> GSHMASDLLEL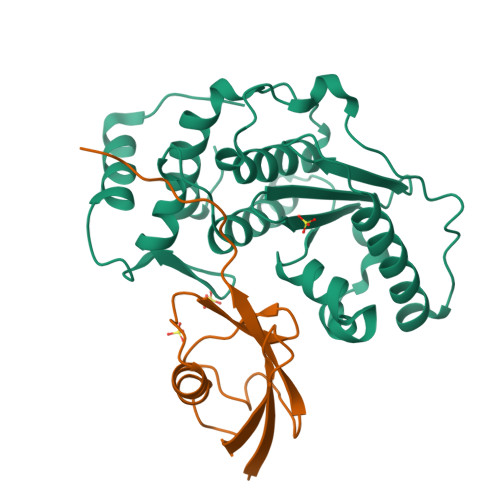TEDMEKEISNALGHGPQDEILSSAFKLRITRGDIQTLKNYHWLNDEVINFYMNLLVERNKKQGYPALHVFSTFFYPKLKSGGYQAVKRWTKGVNLFEQEIILVPIHRKVHWSLVVIDLRKKCLKYLDSMGQKGHRICEILLQYLQDESKTKRNSDLNLLEWTHHSMKPHEIPQQLNGSDSGMFTCKYADYISRDKPITFTQHQMPLFRKKMVWEILHQQLL;> MANDHINLKVAGQDGSVVQFKIKRHTPLSKLMKAYCERQGLSMRQIRFRFDGQPINETDTPAQLEMEDEDTIDVFQQQTGGVYLEHHHHHH The NpnN, Ap4A, Ap5A and Gp4G levels within cells are primarily maintained by Nudix hydrolase superfamily member Ap4A hydrolase (Ap4AH from hereon). Based on sequence analysis the P. falciparum Ap4AH (PfAp4AH, EC 3.6.1.17) was predicted to be an animal-archeal type which cleaves polyphosphate chain at the fourth phosphate from the tightly bound adenosine resulting in asymmetrical cleavage of Ap4A. PfAp4AH can asymmetrically hydrolase Ap4A and Ap5A molecules produced by PfKRS (and probably by other Pf aaRSs) to ATP + AMP and ATP + ADP, respectively. PfAp4AH folds into a conventional Nudix domain, with four β-strands (β1, β2, β4 and β5) sandwiched inside two anti-parallel helices (α1 and α3).

We also provide two crystal structures of PfAp4AH - in apo and sulphate-bound forms at atomic resolution. PfAp4AH apoenzyme (PfAp4AH-apo from hereon) and suphate bound PfAp4AH (PfAp4AH-SO4 from hereon) structures were solved using PHASER MR35 and one chain of iodide-SAD structure was used as template. There are four molecules in asymmetric unit for PfAp4AH-apo and designated as A, B, C and D. The atomic resolution structure of PfAp4AH-SO4 has three SO4 ions and a PEG molecule which arise from crystallization buffer. Global structural differences between apo- and SO4- bound PfAp4AH were apparent upon superimposition. Three major variable regions arising from SO4 binding and different space group packing of PfAp4AH were identified in loop regions L2, L3 and L5 and analyzed further. We were able to solve crystal structure of PfAp4AH in two conformations. These two structures were compared and global changes were mapped for understanding the substrate induced changes.

>MKINIIKAFGILLCRLKKYNPVTTGDINKFEFLFLKASYADKHWTPPKGLHENNESGLETAVRETLEETGINKDKYKLLNYQKTLKYNVKDKPKETTYYLAMLLNNEENVILSDEHTDYKWIGSHESDTYNLPESLADLLKEAEEFLNKEQL[4x]> GAGKQNEVELVAEKQLAFPLDEQTYYLSKSMFQFEENGKEYLHFENTQKSLYDIVIFDIENQQIAKRIPLHKTGPNGLPAVFGSRPSPDSQ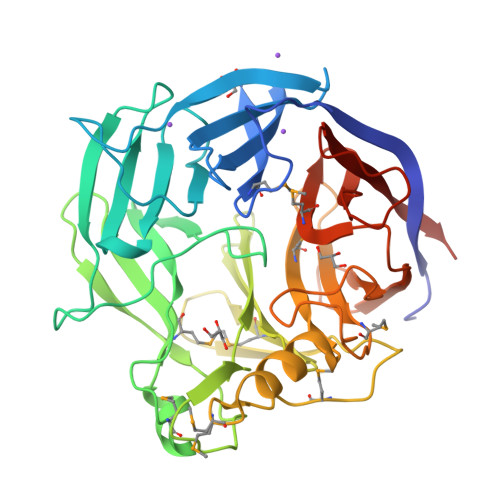YILVAQNNISRLSSINSQGEIIRNYNFQTPEGRFTPLSFGSYYNAPAFIKDSCIFLRQEILKPDMKKEDWPRTHMFASQDLRTGEVKWIPIFYPPIFKEEYDNIAGGYGFSYDYNYKESRLVCGFFGYDSLMVTDDLKHIRWYNAKSRYLKSMKPKLGNSMEGINAIIKLNENPRYWHIMYDKYRNVYYRFAEMPYKLAPNESPYETPKGKEFSVIVLNADFEIIGETKFPGKKYFYKMSFVGREGLYISENNLENPQFDENKLVFTCFKIKNASPNK As an inhibitor of RNase E, RraA has widespread effects on transcript levels in E. coli, although its physiological role in ribonuclease regulation is debated. Surprisingly, in vitro RraA does not inhibit the catalytic activity of RNase E directly, but appears to act indirectly by occluding RNA binding regions in the C-terminal domain of the ribonuclease. We have previously shown that RraA can directly interact with RhlB, and it is possible that RraA plays two distinct roles in modulating the degradosome, by inhibiting both its ribonuclease and helicase activities. We present biochemical and structural data to characterize the interaction between RraA and SrmB, and provide structural data on the interaction of RhlB with RraA and compare the two complexes.

Unlike the interaction between RraA and SrmB, the complex formed between RraA and RhlB appears to be mediated entirely by the CTE of RhlB. Despite extensive efforts we were unable to co-crystallize RraA with full-length RhlB, however, it was possible to obtain co-crystals of RraA with a peptide corresponding to the RhlB CTE (RhlB(398–421)). The structure of RhlB(398–421)/RraA was solved at 2.8-Å resolution, and reveals 12 protomers of RraA in the asymmetric unit of the crystal, organized as stacked trimers that generate two hexamers. The hexameric form of RraA may be a favored oligomerization state at higher protein concentrations, as hexameric assemblies also occur in the crystal structure of isolated RraA. Poorer quality electron density was identified on the surface of a single RraA protomer that is able to accommodate a single RhlB(398–421) peptide. Due to the poor quality of the density it was not possible to model amino acid side chains for the peptide, but 15 of 23 main chain residues could be traced with confidence (two chains of 6 and 9 residues). The density is located close to electronegative patches on the RraA surface, which is compatible with the complementary electropositive nature of RhlB(398–421) (predicted pI 12.5). Nonetheless, the structure indicates an approximate site of RhlB fragment binding on the surface of RraA. Surprisingly, the contact site overlaps with the interface identified for the SrmB/RraA assembly and the modeled RhlB residues lay in proximity of RraA residues Asp-50 and Asp-128. In the proposed model for inhibition of RhlB, the RraA would not contact the RNA binding sites located in the helicase core as it does in the case of SrmB, but instead sequester the CTE.

>[12x]MKYDTSELCDIYQEDVNVVEPLFSNFGGRASFGGQIITVKCFEDNGLLYDLLEQNGRGRVLVVDGGGSVRRALVDAELARLAVQNEWEGLVIYGAVRQVDDLEELDIGIQAMAAIPVGAAGEGIGESDVRVNFGGVTFFSGDHLYADNTGIILSEDPLDIE>GMSTSAIDPVSFSLYAKDFTRFAQELGASFERYGFAVLSDYDLDQARIDAAVDSAK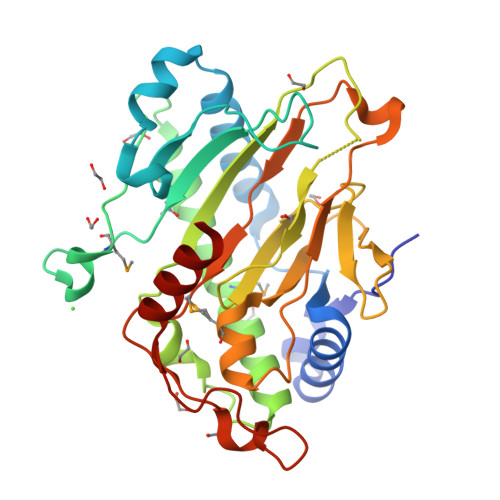AFFALPVETKKQYAGVKGGARGYIPFGVETAKGADHYDLKEFWHMGRDLPPGHRFRAHMADNVWPAEIPAFKHDVSWLYNSLDGMGGKVLEAIATYLKLERDFFKPTVQDGNSVLRLLHYPPIPKDATGVRAGAHGDINTITLLLGAEEGGLEVLDRDGQWLPINPPPGCLVINIGDMLERLTNNVLPSTVHRVVNPPPERRGVPRYSTPFFLHFASDYEIKTLQNCVTAENPDRYPESITADEFLQQRLREIKLA[2x]>MSEPESLMGKLTTHILDLTCGKPAANVKIGLKRLGESIMKEVYTNNDGRVDVPLLAGEELMSGE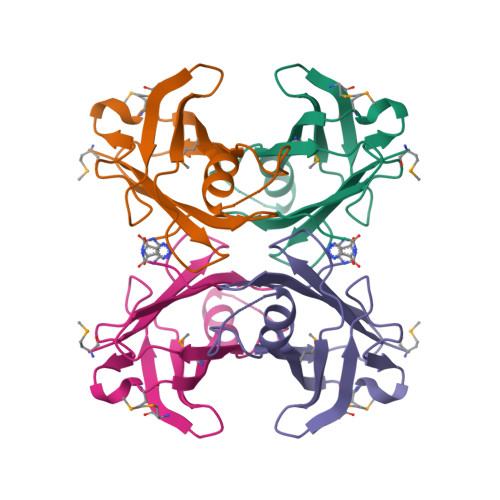YVMEFHAGDYFASKNMNAADQPFLTIVTVRFQLADPDAHYHIPLLLSPFGYQVYRGS[2x]>GSHMEAVQNRIVEAAERVPGVRGVIHLRARYVGQDIWADMIIGVDPENTVEQAHEICEAVQAAVCGKIRRIESLHVSADAREIGDT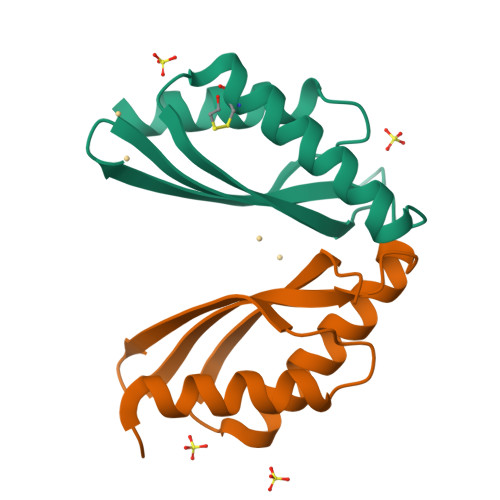TKPSFSDQPLSFDEVMLSKVDN[7x]> MRRVRDGLFLSHPSSALQCSVAVVSTGEFDHPPFQFRQRHTFNTTPLHDANRFGGRTAYLREIGPVNIKKQGRRF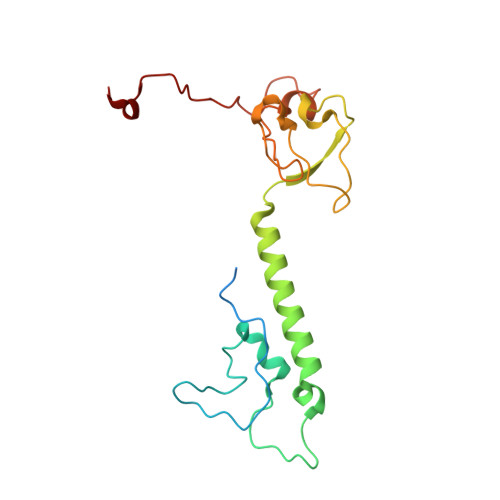KKDPRTVQFNVDVWCAQQTLRKRWKQRDWEVIEIPFRLVPREQQRVIPELYTDIPQMTDPARNDFSNIRNKVYDREELQGVLFPAAGAMLYPPLQRVDKQAMTLDKYL>GAMVKSENLSTGNALIDNELDIRGLFRLLWRGKVWPIAIGLLFAVVALGYSYLVKQEWGATSITDKPTVNMLGGYYSQQQFLRNLDARSFSSPQPEQPSISAGAYDEFIMQLAAYDTRRDFWLQTDYYKQRLEGDEKADAALLDELVNNIQFTARDDGKKTNDSVKLVAETSSDSNTLLRQYVVFASQRAANHLNEEIKGAWAARTIFMKSQIKRQEAVAKAIYDREVRSVELALKIAQQQGISRSQTDTPADEIPASEMFLLGRPMLQARLETLQTSGPHYELDYDQNRAMLATLNVGPTLEASFQTYRYLRTPEEPVKRDSPRRAFLMVMWGAIGVLVGAGVALARRLR[8x]

The enterobacterial common antigen (ECA) is a carbohydrate polymer that is associated with the cell envelope in the Enterobacteriaceae. ECA contains a repeating trisaccharide which is polymerized by WzyE, a member of the Wzy membrane protein polymerase superfamily. WzyE activity is regulated by a membrane protein polysaccharide co-polymerase, WzzE. Wzz proteins consist of two transmembrane helices flanking a large periplasmic domain; there is no cytoplasmic domain.

The 3.6 Å cryo-EM structure of full length WzzEPA that is found as an octamer with a large enclosed central periplasmic lumen connected to a membrane cavity defined by the transmembrane helices. The reconstructed 3D map shows only WzzEPA and that WzzEPA forms an octamer made up of four dimers arranged in C4 symmetry. A prominent conserved feature of the Wzz monomer is a long (approx. 100 Å) helix, which is approximately parallel to the long axis of the molecule. This helix is connected by a helical turn-containing loop (residues 241–265) to two shorter α-helices, which are arranged approximately anti-parallel to the long helix. In the octamer, there are slight structural differences between the monomers localized at the loop that connects the long helix to the two shorter α-helices and this resulted in C4 symmetry. These helices connect to a region of structure identified as motif 1, which is formed by residues 58–204 and 310–317. In WzzEPA, motif 1 consists of a β-sheet with four anti-parallel β-strands and four α-helices. Two regions within motif 1, a loop (residues 153–163) (L-loop) and a loop–helix–loop (78–100), point into the large central periplasmic lumen. The transmembrane helices, which are not closely packed, enclose the disc-shaped cavity within the membrane resembling that seen for other Wzz structures. The location of the antibody indicated that WzyEPA is positioned in the centre of the transmembrane cavity formed by the transmembrane helices of octameric WzzEPA.>DPGTIVHNFSRTEPRTEPAGGSHSGSSSKLQALFAHPLYNVPEEPPLLGAEDSLLASQE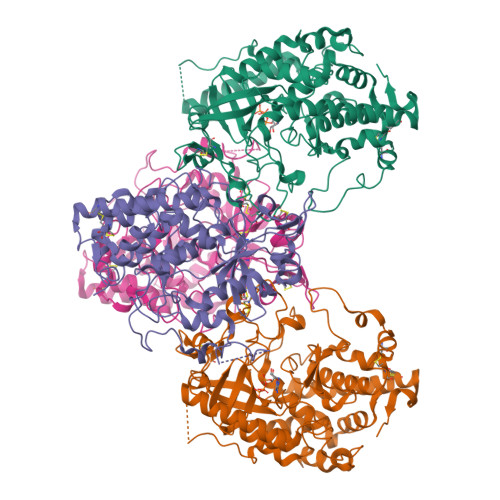ALRYYRRKVARWNRRHKMYREQMNLTSLDPPLQLRLEASWVQFHLGINRHGLYSRSSPVVSKLLQDMRHFPTISADYSQDEKALLGACDCTQIVKPSGVHLKLVLRFSDFGKAMFKPMRQQRDEETPVDFFYFIDFQRHNAEIAAFHLDRILDFRRVPPTVGRIVNVTKEILEVTKNEILQSVFFVSPASNVCFFAKCPYMCKTEYAVCGKPHLLEGSLSAFLPSLNLAPRLSVPNPWIRSYTLAGKEEWEVNPLYCDTVKQIYPYNNSQRLLNVIDMAIFDFLIGNMDRHHYEMFTKFGDDGFLIHLDNARGFGRHSHDEISILSPLSQCCMIKKKTLLHLQLLAQADYRLSDVMRESLLEDQLSPVLTEPHLLALDRRLQTILRTVEGCIVAHGQQSVIVDGPVEQ[2x];>MILFRKFRVLILTVFLIACTMHIMIDLLPKLEKRAAGSSSSAGGGSGCSCAHTPGEEPRSWGKQRARAADPGWPNKHSLRLLQDFSNEPNSNLTSQSREKVTERAGSEKQGSGKRGLMREADSRQRRTDVRVSSVLQSLFEHPLYRTVLPDLTEEDTLFNLNAEIRLYPKAAGQQEWHNEGNVEEEEFSPPGEANSESYPNWLRFHIGINRYELYSRHNPVIAALLRDLLSQKISSVGMKSGGTQLKLIMSFQNYGQALFKPMKQTREQETPPDFFYFSDFERHNAEIAAFHLDRILDFRRVPPVAGRLVNMTREIRDVTRDKKLWRTFFVSPANNICFYGECSYYCSTEHALCGKPDQIEGSLAAFLPDLALAKRKTWRNPWRRSYHKRKKAEWEVDPDYCDEVKQTPPYDRGTRLLDIMDMTIFDFLMGNMDRHHYETFEKFGNDTFIIHLDNGRGFGKHSHDEMSILVPLTQCCRVKRSTYLRLQLLAKEEYKLSSLMEESLLQDRLVPVLIKPHLEALDRRLRLVLKVLSDCVEKDGFSAVVENDLDGQPSVHGGR[2x]>SQAEEDSLDVKDHKLLLFQEVTGLISTWVTSIVEEADWDFERALKLFIQKNADHEIPDLAFAKLGSHMNTVNLSKADKRSLAVARAELVLEQIQQKAN[4x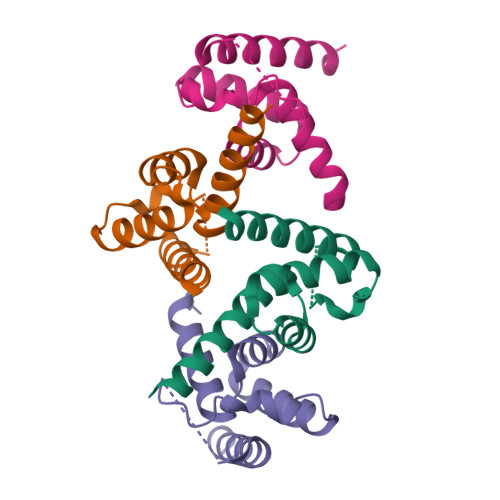]>[4x]MAVTNVAELNALVERVKKAQREYASFTQEQVDKIFRAAALAAADARIPLAKMAVAESGMGIVEDKVIKNHFASEYIYNAYKDEKTCGVLSEDDTFGTITIAEPIGIICGIVPTTNPTSTAI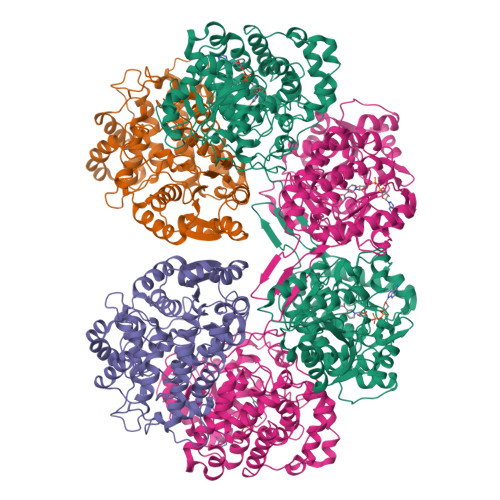FKSLISLKTRNAIIFSPHPRAKDATNKAADIVLQAAIAAGAPKDLIGWIDQPSVELSNALMHHPDINLILATGGPGMVKAAYSSGKPAIGVGAGNTPVVIDETADIKRAVASVLMSKTFDNGVICASEQSVVVVDSVYDAVRERFATHGGYLLQGKELKAVQDVILKNGALNAAIVGQPAYKIAELAGFSVPENTKILIGEVTVVDESEPFAHEKLSPTLAMYRAKDFEDAVEKAEKLVAMGGIGHTSCLYTDQDNQPARVSYFGQKMKTARILINTPASQGGIGDLYNFKLAPSLTLGCGSWGGNSISENVGPKHLINKKTVAKRAENMLWHKLPKSIYFRRGSLPIALDEVITDGHKRALIVTDRFLFNNGYADQITSVLKAAGVETEVFFEVEADPTLSIVRKGAELANSFKPDVIIALGGGSPMDAAKIMWVMYEHPETHFEELALRFMDIRKRIYKFPKMGVKAKMIAVTTTSGTGSEVTPFAVVTDDATGQKYPLADYALTPDMAIVDANLVMDMPKSLCAFGGLDAVTHAMEAYVSVLASEFSDGQALQALKLLKEYLPASYHEGSKNPVARERVHSAATIAGIAFANAFLGVCHSMAHKLGSQFHIPHGLANALLICNVIRYNANDNPTKQTAFSQYDRPQARRRYAEIADHLGLSAPGDRTAAKIEKLLAWLETLKAELGIPKSIREAGVQEADFLANVDKLSEDAFDDQCTGANPRYPLISELKQILLDTYYGRDYVEGETAAKKEAAPAKAEKKAKKSA>[2x]GRNADRKQILGIPKLDDANEAGGKYSHRCTLILTEGDSAKALCTAGLAVKDRDYFGVFPLRGKPLNVRDATLKKVMACAEFQAVSKIMGLDIRQKYSGVERLRYGHLMIMSDQDHDGSHIKGLIINMIHHYWPDLIKTPGFLQQFITPIVKARKKGRSDGDDRAISFFSMPDYFEWKNAIGDGIRNYEIRYYKGLGTSGAKEGREYFENIDR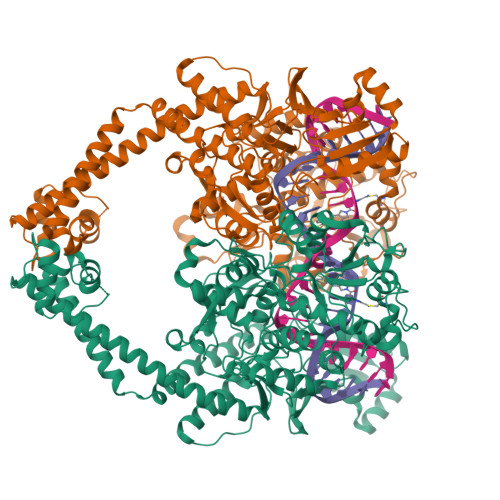HRLDFVHEDATDDARIVMAFAKDKVEERKHWITQFKANTNVNESMNYNVRTVRYSEFVDKELILFSVADCERSIPSVIDGLKPGQRKIIFSSFKRRLTRSIKVVQLAGYVSEHAAYHHGEQSLVQTIVGLAQNFVGSNNVPLLQQDGQFGTRLQGGKDHAAGRYIFTRLTNIARYIYHPSDDFVVDYKDDDGLSVEPFYYVPVIPMVLVNGTSGIGTGFATNIPNYSPLEVIDNLMRLLRGEEVQPMKPWYFGFAGTIEEKEKGKFVSTGCANVRPDGVVQITELPIGTWTQGYKKFLEELREKEVVVQYREHNTDVTVDFEVFLHPEVLHHWVAQGCVEERLQLREYIHATNIIAFDREGQITKYRDAEAVLKEFYLVRLEYYAKRRDFLIGDLRSVASKLENMVRFVTEVVDGRLIVTRRRKKELLEELRQRGYAPFPLQQKKKVSSTTIQQGEEEGAADATHATAEDVFLVLQPAVDEGGDEDNQETPEMRRAARDYDYLLGMRLWNLTAEMIARLQSQLQKARDELAALEKRTPKDLWAEDLNQLRPRIENLFEERAKEIASI>HMSVGIVYGDQYRQLCCSSPKFGDRYALVMDLINAYKLIPELSRVPPLQWDSPSRMYEAVTAFHSTEYVDALKKLQMLHCEEKELTADDELLMDSFSLNYDCPGFPSVFDYSLAAVQGSLAAASALICRHCEVVINWGGGWHHAKRSEASGFCYLNDIVLAIHRLVSSTPPETSPNRQTRVLYVDLDLHHGDGVEEAFWYSPRVVTFSVHHASPGFFPGTGTWNMVDNDKLPIFLNGAGRGRFSAFNLPLEEGINDLDWSNAIGPILDSLNIVI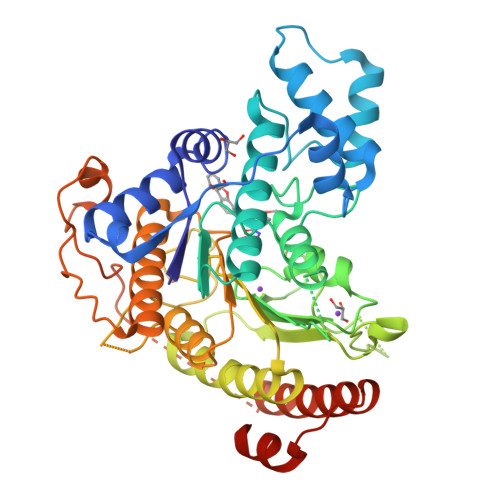QPSYVVVQCGADCLATDPHRIFRLTNFYPNLNLDSDCDSECSLSGYLYAIKKILSWKVPTLILGGGGYNFPDTARLWTRVTALTIEEVKGKKMTISPEIPEHSYFSRYGPDFELDIDYFPHESHNKTLDSIQKHHRRILEQLRNYADLNKLIYDYDQVYQLYNLTGMGSLVPR[4x]NA, which is a sialidase, catalyzes hydrolysis of terminally linked sialic acid and functions as the receptor-destroying element of influenza A and B viruses. Additionally, influenza A NA is further classified into two groups: group 1 (N1, N4, N5 and N8) and group 2 (N2, N3, N6, N7 and N9), based upon primary sequence. Group 1 NAs contain a 150-cavity (formed by amino acids 147–151 of the 150-loop) in their active site, whereas group 2 NAs lack this cavity. NA inhibition assays were carried out and complex crystal structures were solved for laninamivir, laninamivir octanoate, zanamivir and oseltamivir in order to elucidate the structural basis of their inhibition.

Therefore, we also solved the p09N1 oseltamivir complex structure at a resolution of 1.7 Å. Binding of oseltamivir to p09N1 was indeed highly similar to the binding observed in previous reports and is also similar to the binding mode of laninamivir octanoate to p09N1. As observed in the other available oseltamivir-NA complex structures, in the p09N1-laninamivir octanoate complex structure, Glu276 indeed forms a salt bridge with Arg224, creating a hydrophobic pocket which accommodates the hydrophobic oseltamivir pentyl ether group. This hydrophobic side chain of oseltamivir is favorably parallel to the Cβ and Cγ of Glu276 on one end and at the other end is pointed toward the hydrophobic Ile222 side chain, which contributes significantly to the high level of oseltamivir inhibition. Oseltamivir contains a 4-amino group, instead of the 4-guanidino group found in zanamivir and laninamivir, and is actually more similar to the natural ligand in this regard. Therefore, the orientation of the 150-loop during oseltamivir binding is not a major factor. Instead, the binding preference of oseltamivir for p09N1 over p57N2 and N5 may be instead explained by the ability of Glu276 to adopt the conformation that is critical to accommodate the osetalmivir pentyl ether side chain, which replaces the glycerol moiety of zanamivir, laninamivir and sialic acid. The observation that this Glu276 conformation occurs in the p09N1-laninamivir octanoate complex, but not the p57N2-laninamivir octanoate complex may indicate that this conformation is more stable in p09N1 after ligand binding which may explain why inhibition of p09N1 by oseltamivir was the best relative to N5 and p57N2. Oseltamivir inhibited the activity of N5, p09N1 and p57N2 with IC50 values of 0.83 nM, 0.54 nM and 0.79 nM, respectively.

>SVKLAGNSSLCPVSGWAIYSKDNSVRIGSKGDVFVIREPFISCSPLECRTFFLTQGALLNDKHSNGTIKDRSPYRTLMSCPIGEVPSPYNSRFESVAWSASACHDGINWLTIGISGPDNGAVAVLKYNGIITDTIKSWRNNILRTQESECACVNGSCFTVMTDGPSNGQASYKIFRIEKGKIVKSVEMNAPNYHYEECSCYPDSSEITCVCRDNWHGSNRPWVSFNQNLEYQIGYICSGIFGDNPRPNDKTGSCGPVSSNGANGVKGFSFKYGNGVWIGRTKSISSRNGFEMIWDPNGWTGTDNNFSIKQDIVGINEWSGYSGSFVQHPELTGLDCIRPCFWVELIRGRPKENTIWTSGSSISFCGVNSDTVGWSWPDGAELPFTIDK[2x]6-[(4-methyl-1,4-diazepan-1-yl)methyl]quinoline | C16 H21 N3 | 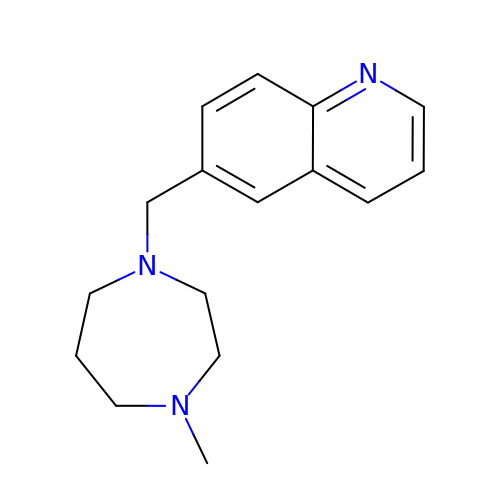DIQRHBUDTKMUNJ-UHFFFAOYSA-N> NVHNTELASSTSENSVETQEITTFHDVETPNRIDTPMAQDTSSARNMDDTHSIIQFLQRPVLIDNIEIIAGTTADANKPLSRYVLDQQNSQKYVRSWTLPSTVLRAGGKAQKLANFKYLRCDVQVKLVLNANPFVAGRMYLAYSPYDDKVDTARSVLQTSRAGVTGYPGVELDF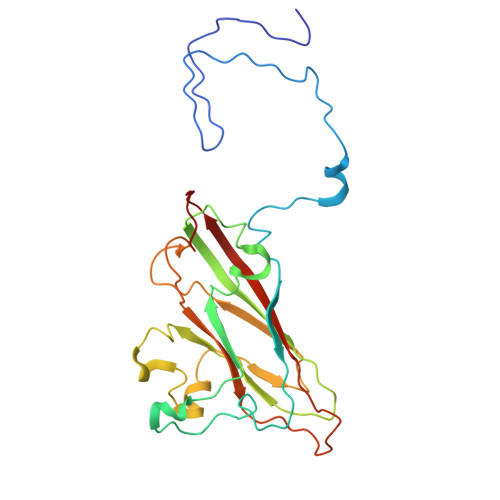QLDNSVEMTIPYASFQEAYDLVTGTEDFVQLYLFPITPVLGPKSESESSKVDISVYMWLSNISLVIPTYRINP> SNAMKTINLSIFGLGNVGLNLLRIIRSFNEENRLGLKFNVVFVADSLHSYYNERIDIGKVISYKEKGSLDSLEYESISASEALARDFDIVVDATPASADGKKELAFYKETFENGKDVVTANKSGLANFWPEIMEYARSNNRRIRYEATVAGGVPLFSFIDYSVLPSRIKKFRGIVSLTINYFIRELANKREFDDVLSEATKLGIVEKNYKDDLTGLDAARKSVILC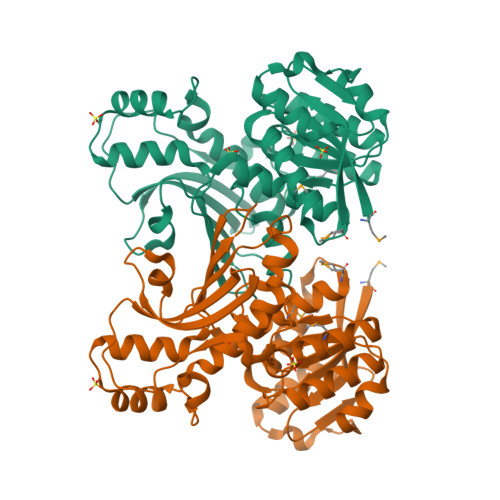NHLYGSSYRLSDVFYEGILDQDRSFGKNERLVTETGIVNGKPSAESRIKSLDSNDYLLTLGKGSLGYQLQTDTNGTLNVSDLYDGPYETAGAVMNDLVILSMFTV The TEC family kinase, BTK (Bruton’s tyrosine kinase) is best known as the target of ibrutinib (IMBRUVICA), the first-in-class covalent kinase active site inhibitor used to treat chronic lymphocytic leukemia, mantle cell lymphoma, Waldenström’s macroglobulinemia, and chronic graft-versus-host disease. The TEC and SRC kinases share the SH3–SH2–kinase domain arrangement (the ‘Src module’). In contrast, BTK contains an extended N-terminal region (PHTH–PRR) consisting of the phospholipid-binding Pleckstrin homology (PH) domain followed by a Tec homology (TH) domain and a long linker housing two proline-rich regions (PRR). Membrane-induced dimerization activates BTK and we present here a crystal structure of an activation loop swapped BTK kinase domain dimer that likely represents the conformational state leading to trans-autophosphorylation. Together, these data provide the first structural elucidation of full-length BTK and allow a deeper understanding of allosteric control over the BTK kinase domain during distinct stages of activation.

With the stabilized full-length BTK mutant showing low activity and a more compact conformational ensemble in solution, we built a full-length BTK construct for crystallization screens that incorporated the 4P1F mutations and the ITK loop. In addition, the catalytic K430 was mutated to arginine to eliminate kinase activity that could produce heterogeneity. The resulting construct, referred to as full-length BTK with stabilized core (FL BTKsc), provided diffraction quality crystals (5–7 days at 4°C) both in the apo form and in the presence of various active site inhibitors. The highest resolution data collected (3.4 Å) was in the presence of the GDC-0853 (fenebrutinib) inhibitor. Despite efforts to stabilize the autoinhibited form, the electron density derived from crystals of full-length BTK (FL BTKsc) defines the same domain swapped dimer observed for the previously solved structure of the BTK SH3–SH2–kinase fragment (Wang et al., 2015). A 16.9° rotation along residues 346–384 in the SH2 and SH2–kinase linker is observed for the domain swapped dimer structure solved here compared to that solved previously. Notably, there is no PHTH domain density visible even after the structure is fully refined. The result shows the crystal is full-length BTK protein with no evidence of smaller BTK fragments. The solvent content in the crystals of full-length BTK is high (67%) and crystal packing shows large solvent channels. The crystallography results are consistent with a flexible N-terminal PHTH domain with the caveat that crystal packing might limit native autoinhibitory contacts between the PHTH and SH3–SH2–kinase regions.

> MAAVILESIFLKRSQQKKKTSPLNFKKRLFLLTVHKLSYYEYDFERGRRGSKKGSIDVEKITCVETVIPEKNPPPERQIPRRGEESSEMEQISIIERFPYPFQVVYDEGPLYVFSPTEELRKRWIHQLKNVIRYNSDLVQKYHPCFWIDGQYLCCSQTAKNAMGCQILENRNGSLKPGSSHRKTKKPLPPTPEEDQILKKPLPPEPTAAPISTTELKKVVALYDYMPMNANDLQLRKGEEYFILEESNLPWWRARDKNGQEGYIPSNYITEAEDSIEMYEWYSKHMTRSQAEQLLKQAGAAGGFIVRDSSKAGKYTVSVFAKSTGEPQGVIRHYVVCSTPQSQYYLAEKHLFSTIPELINYHQHNSAGLISRLKYPVSKQNKNPPPPPGFGYGSWEIDPKDLTFLKELGTGQFGVVKYGKWRGQYDVAIRMIREGSMSEDEFIEEAKVMMNLSHEKLVQLYGVCTKQRPIFIITEYMANGCLLNYLREMRHRFQTQQLLEMCKDVCEAMEYLESKQFLHRDLAARNCLVNDQGVVKVSDFGMTRYVLDDEYTSSTGSKFPVKWASPEVLMYSKFSSKSDIWAFGVLMWEIYSLGKMPYERFTNSETAEHIAQGLRLPRPHLASERVYTIMYSCWHEKADERPSFKILLSNILDVMDEES> MVSAIVLYVLLAAAAHSAFALQDPCSNCPAGTFCDNNRNQICSPCPPNSFSSAGGQRTCDICRQCKGVFRTRKECSSTSNAECDCTPGFHCLGAGCSMCEQD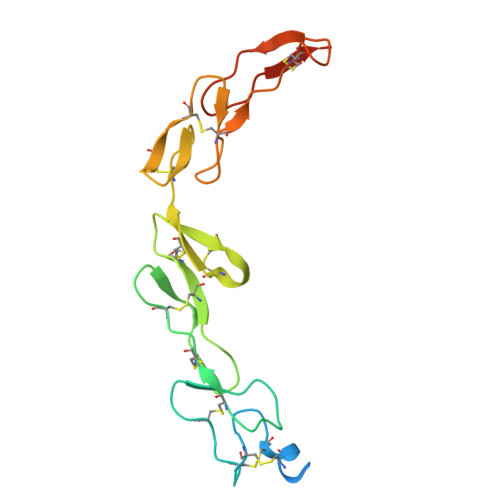CKQGQELTKKGCKDCSFGTFNDQKRGICRPWTDCSLDGKSVLVDGTKERDVVCGPGSHHHHHH> DNLEQKILQVLSDDGGPVKIGQLVKKCQVPKK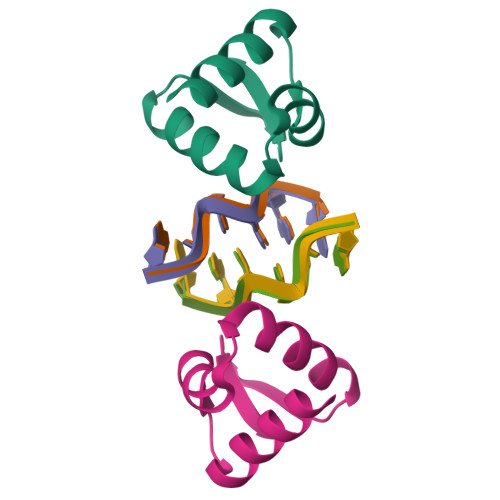TLNQVLYRLKKEDRVSSPEPATWSIGG> MHHHHHHGENLYFQGSGSVSSGQAHSLASLAKTWSSGSAKLQRLGPETEDNEGVLLTEKLKPVDYEYREEVHWMTHQPRLGRGSFGEVHRMKDKQTGFQCAVKKVRLEVFRVEELVACAGLSSPRIVPLYGAVREGPWVNIFMELLEGGSLGQLIKQMGCLPEDRALYYLGQALEGLEYLHTRRILHGDVKADNVLLSSDGSRAALCDFGHALCLQPDGLGKSLLTGDYIPGTETHMAPEVVMGKPCDAKVDIWSSCCMMLHMLNGCHPWTQYFRGPLCLKIASEPPPIR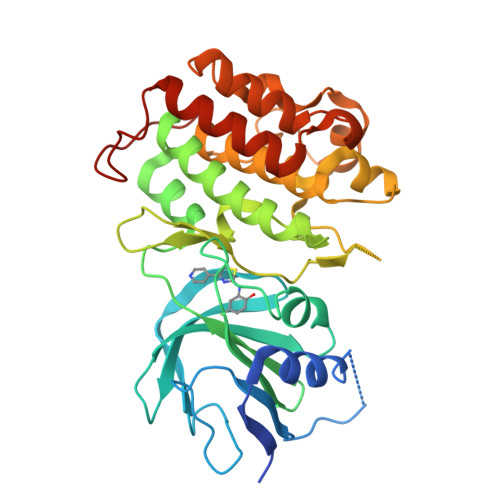EIPPSCAPLTAQAIQEGLRKEPVHRASAMELRRKVGKALQEVGGLKSPWKGEYKEPRGNS> AEKLFTPLKVGAVTAPNRVFMAPLTRLRSIEPGDIPTPLMGEYYRQRASAGLIISEATQISAQAKGYAGAPGLHSPEQIAAWKKITAGVHAEDGRIAVQLWHTGRISHSSIQPGGQAPVSASALNANTRTSLRDENGNAIRVDTTTPRALELDEIPGIVNDFRQAVANAREAGFDLVELHSAHGYLLHQFLSPSSNQRTDQYGGSVENRARLVLEVVDAVCNEWSADRIGIRVSPIGTFQNVDNGPNEEADALYLIEELAKRGIAYLHMSETDLAGGKPYSEAFRQKVRERFHGVIIGAGAYTAEKAEDLIGKGLIDAVAFGRDYIANPDLVARLQKKAELNPQRP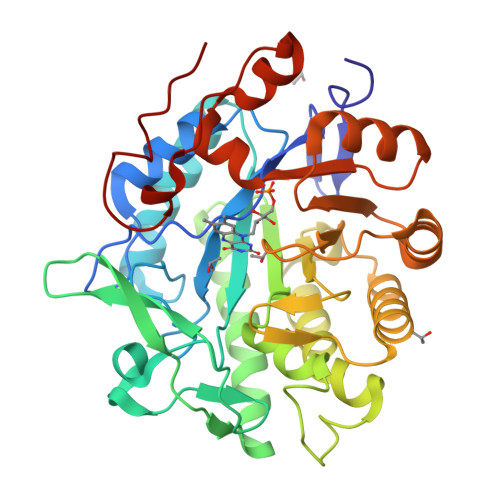ESFYGGGAEGYTDYPSL> MWATLPLLCAGAWLLGVPVCGAAELC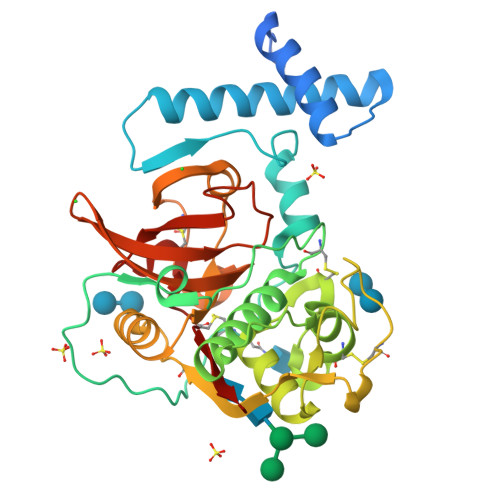VNSLEKFHFKSWMSKHRKTYSTEEYHHRLQTFASNWRKINAHNNGNHTFKMALNQFSDMSFAEIKHKYLWSEPQNCSATKSNYLRGTGPYPPSVDWRKKGNFVSPVKNQGACGSSWTFSTTGALESAIAIATGKMLSLAEQQLVDCAQDFNNHGCQGGLPSQAFEYILYNKGIMGEDTYPYQGKDGYCKFQPGKAIGFVKDVANITIYDEEAMVEAVALYNPVSFAFEVTQDFMMYRTGIYSSTSCHKTPDKVNHAVLAVGYGEKNGIPYWIVKNSWGPQWGMNGYFLIERGKNMCGLAACASYPIPLV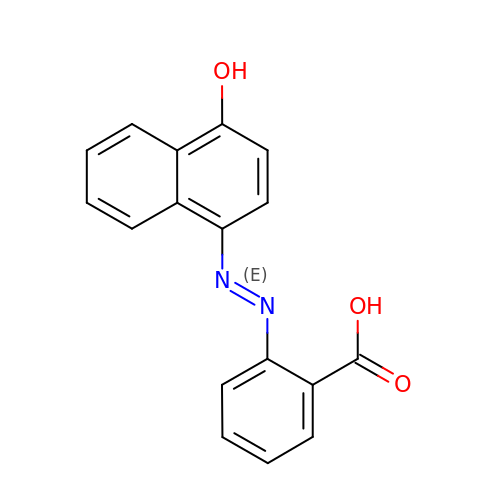2-((4'-HYDROXYNAPHTHYL)-AZO)BENZOIC ACID | C17 H12 N2 O3 | SXAUIPSOPPASFY-VHEBQXMUSA-N> GSHMQDPEQLKHCNGILKELLSKKHAAYAWPFYKPVDASALGLHDYHDIIKHPMDLSTVKRKMENRDYRDAQEFAADVRLMFSNCYKYNPPDHDVVAMARKLQDVFEFRYAKMPA

The BET family proteins (BRD2, BRD3, BRD4, and BRDT) contain two tandem bromodomains and an extra-terminal domain at the C-terminal. The BET family proteins generally recognize acetylated histones H3 and H4 (and references therein); however, BRD2 preferentially recognize mono/di-acetylated histone tail of H4. The tertiary structure of all bromodomains contains a left-handed α-helical bundle formed by four α-helices (αZ, αA, αB, and αC). The α-helical bundle along with flanking ZA and BC loops create a deep hydrophobic cavity, which recognizes a specific sequence of acetylated-histone tails.

Here, we discuss a newly identified small molecule inhibitor (NSC127133; hereafter, L10), a phenanthridinone derivative, of the second bromodomain (BD2) of BRD2. The BD2-L10 crystals diffracted to an atomic resolution of 0.91 Å resolution in P22121 space group, with one molecule per asymmetric unit. The L10 compound, which binds in the deep hydrophobic cleft, is surrounded by the amino acids P371, V376, L381, L383, Y386, N429, H433 and V435. The phenanthridinone moiety, which sits in the deep cleft, is stabilized by both hydrophobic as well as by several direct and water mediated hydrogen bond interactions. One important feature of L10 binding to BD2 is the direct double hydrogen bonds of phenanthridinone O9 and N9 atoms to the carboxamide side chain of N429. Moreover, the O9 atom of L10 is also hydrogen bonded to a conserved water molecule W3 (2.92 Å), which forms a three-way hydrogen bond to the backbone amino and carbonyl group of C425 and N424, respectively, and to the sidechain hydroxyl group of Y386. The carbamoyl moiety, which links the phenanthridinone and phenyl-benzoic acid group, makes direct electrostatic interactions with NE2 of H433. The phenyl-benzoic acid moiety protrudes away from the binding site and does not have any interactions with the BD2 protein. As speculated, the ligand L10 binds significantly well with BRD2-BD2 and the dissociation constant (KD) estimated by globally fitting the equilibrium state response observed at different L10 concentrations is 213.7 μM. Superposition of the BD2-L10 and BD2-H4K5ac complex structures reveals that the binding of phenanthridinone ring moiety of L10 mimics the Kac binding with the BD2.>[2x]MVSGFAMPKIWRKLAMDIPVNAAKPGRRRYLTLVMIFITVVICYVDRANLAVASAHIQEEFGITKAEMGYVFSAFAWLYTLCQIPGGWFLDRVGSRVTYFIAIFGWSVATLFQGFATGLMSLIGLRAITGIFQAPAFPTNNRMVTSWFPEHERASAVGFYTSGQFVGLAFLTPLLIWIQEMLSWHWVFIVTGGIGIIWSLIWFKVYQPPRL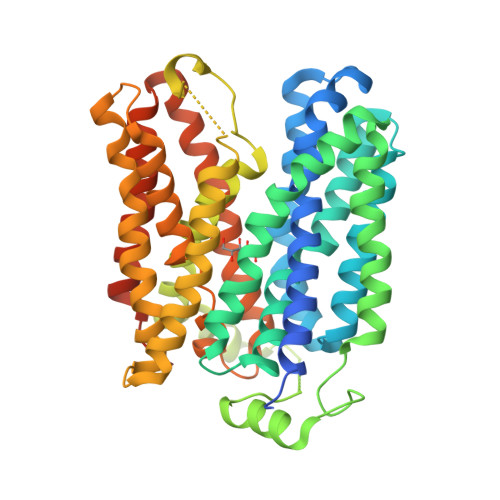TKGISKAELDYIRDGGGLVDGDAPVKKEARQPLTAKDWKLVFHRKLIGVYLGQFAVASTLWFFLTWFPNYLTQEKGITALKAGFMTTVPFLAAFVGVLLSGWVADLLVRKGFSLGFARKTPIICGLLISTCIMGANYTNDPMMIMCLMALAFFGNGFASITWSLVSSLAPMRLIGLTGGVFNFAGGLGGITVPLVVGYLAQGYGFAPALVYISAVALIGALSYILLVGDVKRVGSLVPRGSGSHHHHHH>[2x]MKMASNDATPSDDGAAGLVPEINNEVMALEPVAGASIAAPVVGQQNIIDPWIRNNFVQAPAGEFTVSPRNSPGELLLDLELGPELNPYLAHLARMYNGHAGGMEVQIVLAGNAFTAGKILFAAIPPSFPYENLSPAQLTMCPHVIVDV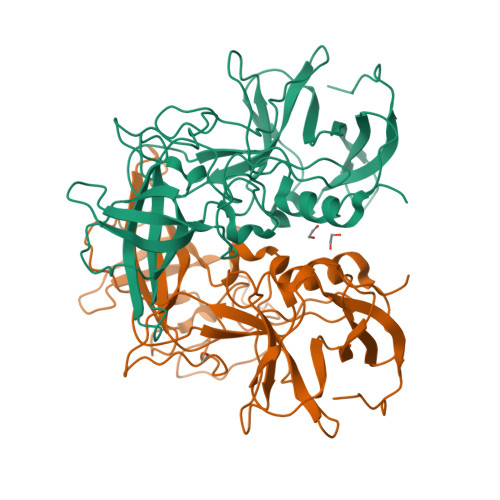RQLEPVLLPMPDIRNVFYHYNQNNSPKLRLVAMLYTPLRANNSGDDVFTVSCRVLTRPSPDFQFTFLVPPTVESKTKNFTLPVLRVSEMTNSRFPVVLDQMYTSRNENIIVQPQNGRCTTDGELLGTTTLQSVSICNFRGTMQAKLNEQPRYQLQLTNLDGSPIDPTDDMPAPLGTPDFQAMLYGVASQRSSRDNATRAHDAQIDTAGDTFAPKIGQVRFKSSSDDFDLHDPTKFTPIGVNVDDQHPFRQWSLPNYGGHLALNNHLAPAVTPLFPGEQILFFRSHIPSAGGHTDGAIDCLLPQEWIEHFYQEAAPSQSDIALVRFINPDTGRVLLEAKLHKQGFLTVAASGDHPIVMPTNGYFRFEAWVNPFYTLAPVGTGSGRRRIQ> MTAVEIIISIFVLIGGFLSLLGSIGIIRFPDVYGRLHAATKSATLGVISIMLATFLFFFLVHGEFVGKLLLTILFVFLT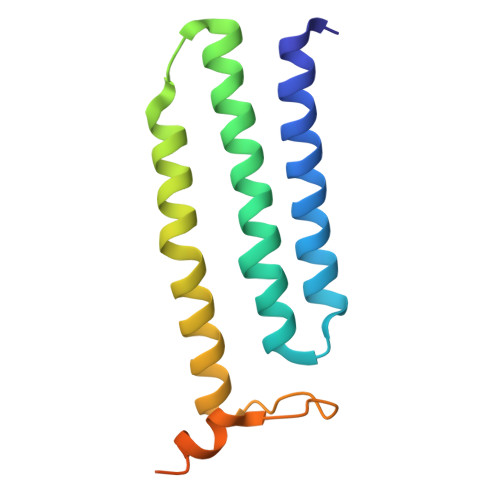APVAGMMMGRSAYRVGVPLWEKSTQDDLKKMYEKKMKGSNHHHHHHDYKDDDDK>MRGSHHHHHHGSAKITTVIDIGSNSVRLAVFKKTSQFGFYLLFETKSKVRISEGCYAFNGILQEIPMQRAVKALSEFKEIALKYKSKKILCVATSAVRDAPNRLEFVARVKKACGLQIKIIDGQKEALYGGIACANLLHKNSGITIDIGGGSTECALIEKGKIKDLISLDVGTIRIKEMFLDKDLDVKLAKAFIQKEVSKLPFKHKNAFGVGGTIRALSKVLMKRFDYPIDSLHGYEIDAHKNLAFIEKIVMLKEDQLRLLGVNEERLDSIRSGALILSVVLEHLKTSLMITSGVGVREGVFLSDLLRNHYHKFPPNINPSLISLKDRFLPHEKHSQKVKKECVKLFEALSPLHKIDEKYLFHLKIAGELASMGKILSVYLAHKHSAYFILNALSYGFSHQDRAIICLLA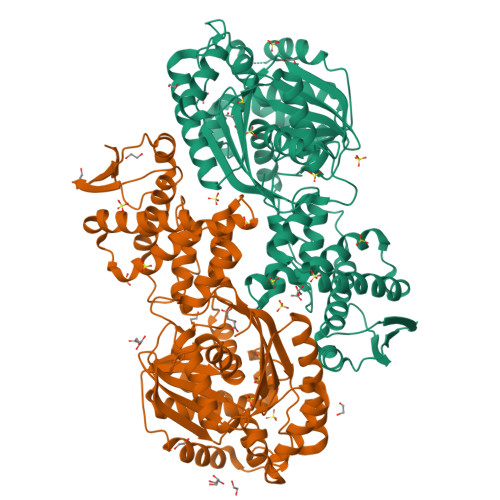QFSHKKIPKDNAIAHMSAMMPSLLTLQWLSFILSLAENLCLTDSHHLKYTLEKNKLVIHSNDALYLAKEMLPKLVKPIPLTIEFA[2x]>QRHITEFISSWQNHPIVQVSADVENKKTAQLLHADTPRLVTWDAGLCTSFKIVPIVPAQVPQDVLAYTFFTSSYAIQSPFPEAAVSRIVVHTRWASNVDFDRDSSVIMAPPTENNIHLFKQLLNTETLSVRGANPLMFRANVLHMLLEFVLDNLY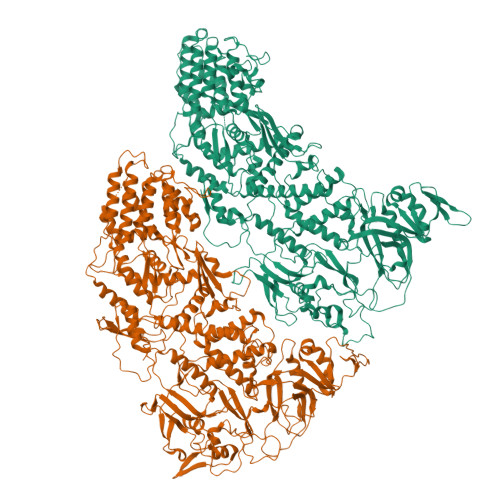LNRHTGFSQDHTPFTEGANLRSLPGPDAEKWYSIMYPTRMGTPNVSKICNFVASCVRNRVGRFDRAQMMNGAMSEWVDVFETSDALTVSIRGRWMARLARMNINPTEIEWALTECAQGYVTVTSPYAPSVNRLMPYRISNAERQISQIIRIMNIGNNATVIQPVLQDISVLLQRISPLQIDPTIISNTMSTVSESTTQTLSPASSILGKLRPSNSDFSSFRVALAGWLYNGVVTTVIDDSSYPKDGGSVTSLENLWDFFILALALPLTTDPCAPVKAFMTLANMMVGFETIPMDNQIYTQSRRASAFSTPHTWPRCFMNIQLISPIDAPILRQWAEIIHRYWPNPSQIRYGAPNVFGSANLFTPPEVLLLPIDHQPANVTTPTLDFTNELTNWRARVCELMKNLVDNQRYQPGWTQSLVSSMRGTLDKLKLIKSMTPMYLQQLAPVELAVIAPMLPFPPFQVPYVRLDRDRVPTMVGVTRQSRDTITQPALSLSTTNTTVGVPLALDARAITVALLSGKYPPDLVTNVWYADAIYPMYADTEVFSNLQRDMITCEAVQTLVTLVAQISETQYPVDRYLDWIPSLRASAATAATFAEWVNTSMKTAFDLSDMLLEPLLSGDPRMTQLAIQYQQYNGRTFNVIPEMPGSVIADCVQLTAEVFNHEYNLFGIARGDIIIGRVQSTHLWSPLAPPPDLVFDRDTPGVHIFGRDCRISFGMNGAAPMIRDETGMMVPFEGNWIFPLALWQMNTRYFNQQFDAWIKTGELRIRIEMGAYPYMLHYYDPRQYANAWNLTSAWLEEITPTSIPSVPFMVPISSDHDISSAPAVQYIISTEYNDRSLFCTNSSSPQTIAGPDKHIPVERYNILTNPDAPPTQIQLPEVVDLYNVVTRYAYETPPITAVVMGVP[2x]In response, one family of large bacteriophages uses a nucleus-like compartment to protect its replicating genomes by excluding host defence factors. Here we find that the bacteriophage nuclear shell assembles primarily from one protein, which we name chimallin (ChmA). Combining cryo-electron tomography of nuclear shells in bacteriophage-infected cells and cryo-electron microscopy of a minimal chimallin compartment in vitro, we show that chimallin self-assembles as a flexible sheet into closed micrometre-scale compartments. We find that the shell is primarily composed of a single protein, chimallin, which self-assembles through its extended N and C termini into a closed compartment.

Localized reconstruction of the square faces from each particle with C4 symmetry resulted in an improved density map at approximately 3.4 Å resolution. Each tetrameric unit in these assemblies is an 11.5 × 11.5 nm square, in line with our in situ subtomogram analysis of the phage nuclear shell. Atomic models of the C4-symmetric chimallin tetramer and quasi-O-symmetric cubic assemblies reveal the molecular basis for chimallin self-assembly. The N-terminal interacting segment (NTS: residues 48–61) of each protomer extends anticlockwise (as viewed from outside the cube) and docks against a neighbouring protomer’s N-terminal domain within a given face of the cubic assembly, thus establishing intra-tetramer connections. To investigate the interconnectivity of chimallin protomers in the context of the phage nucleus, we docked copies of the high-resolution chimallin tetramer model into the in situ cryo-ET map. The chimallin tetramers fit well into the 24 Å-resolution cryo-ET map of the shell without clashes and with an overall map–model correlation coefficient of 0.56. Docking the tetramer model into maps representing concave, flat, and convex subpopulations indicated that the best fit is to the convex class (model–map correlation coefficient = 0.64), and the worst fit is to the concave class (model–map correlation coefficient = 0.51). The tetramer model derived from the cubic assembly, which represents a highly convex state, shows a further approximately 25° inward tilt of each protomer. These observations suggest that the chimallin tetramer itself is flexible, with the C-terminal domains on the shell’s inner face rotating inward in convex regions of the shell, and outward in concave regions.

>SNAMIRDTATNTTQTQAAPQQAPAQQFTQAPQEKPMQSTQSQPTPSYAGTGGINSQFTRSGNVQGGDARASEALTVFTRLKEQAVAQQDLADDFSILRFDRDQHQVGWSSLVIAKQISLNGQPVIAVRPLILPNNSIELPKRKTNIVNGMQTDVIESDIDVGTVFSAQYFNRLSTYVQNTLGKPGAKVVLAGPFPIPADLVLKDSELQLRNLLIKSVNACDDILALHSGERPFTIAGLKGQQGETLAAKVDIRTQPLHDTVGNPIRADIVVTTQRVRRNGQQENEFYETDVKLNQVAMFTNLERTPQAQAQTLFPNQQQVATPAPWVASVVITDVRNADGIQANTPEMYWFALSNAFRSTHGHAWARPFLPMTGVAKDMKDIGALGWMSALRNRIDTKAANFDDAQFGQLMLSQVQPNPVFQIDLNRMGETAQMDSLQLDAAGGPNAQKAAATIIRQINNLGGGGFERFFDHTTQPILERTGQVIDLGNWFDGDEKRDRRDLDNLAALNAAEGNENEFWGFYGAQLNPNLHPDLRNRQSRNYDRQYLGSTVTYTGKAERCTYNAKFIEALDRYLAEAGLQITMDNTSVLNSGQRFMGNSVIGNNMVSGQAQVHSAYAGTQGFNTQYQTGPSSFY[12x]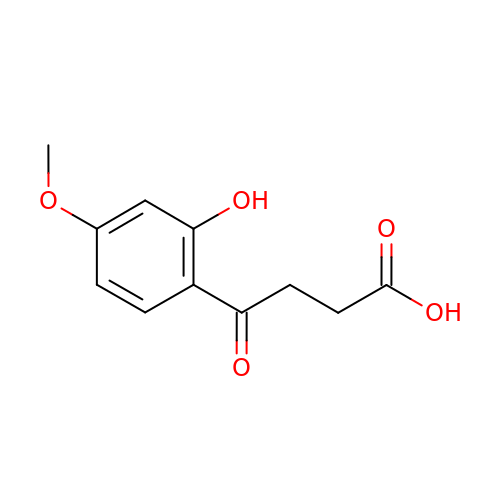4-(2-hydroxy-4-methoxyphenyl)-4-oxobutanoic acid | C11 H12 O5 | MMMHZBODZRNHIN-UHFFFAOYSA-N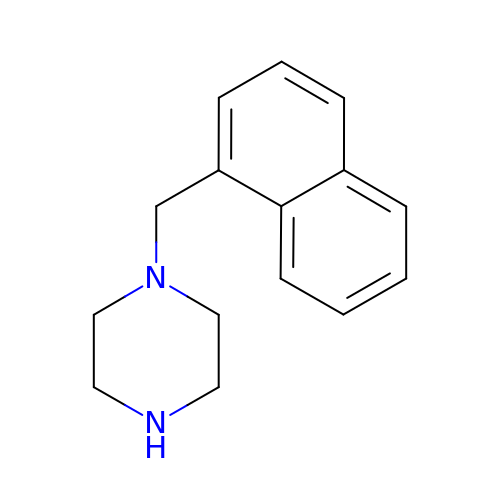1-(naphthalen-1-ylmethyl)piperazine | C15 H18 N2 | HGYDREHWXXUUIS-UHFFFAOYSA-N Outer mitochondrial membrane (OMM) fusion is catalyzed by the dynamin-like GTPase called mitofusin (MFN). We generated a modified human MFN2 construct with deletions of residues 1–21 and 401–705 (MFN2IM). MFN2IM contains a G domain and a helical domain 1 (HD1). In this study, we address these issues by presenting crystal structures of truncated human MFN2 in different stages of the GTP turnover cycle. These structures explain how MFN2 uses a primate-only single amino acid variance and a tighter G interface, as compared with human MFN1, to allow for enduring GTPase (G) domain association even after GTP hydrolysis, a feature that is unique in the dynamin superfamily and ensures efficient membrane tethering.

To investigate how Thr111 phosphorylation affects the function of MFN2, we solved the crystal structure of a phosphorylation mimic MFN2IM(T111D). According to the structure, the side chain of Asp111 is not fully exposed, and its phosphorylation may require a substantial local conformational rearrangement. Phosphorylated Thr111, as reflected by the Asp111 in the crystal structure, blocks the binding groove for GTP in the P-loop, and the negative charge is also disfavored for the phosphate groups of the nucleotide. Subsequent ITC analysis confirmed that MFN2IM(T111D) has no binding affinity to guanine nucleotides. Therefore, the putative phosphorylation at Thr111 is likely to directly inactivate MFN2 in mediating mitochondrial fusion. Intriguingly, we observed calcium ions (Ca2+) associated with the HD1 of both nucleotide-free wild-type MFN2IM and MFN2IM(T111D), and one of them is involved in intermolecular contact. Addition of Ca2+ did not alter the biochemical features of wild-type MFN2IM or MFN2IM(T111D).

>GPHMGGSAEVNASPLKHFVTAKKKINGIFEQLGAYIQESATFLEDTYRNAELDPVTTEEQVLDVKGYLSKVRGISEVLARRHMKVAFFGRTSNGKSDVINAMLWDKVLPSGIGHTTNCFLRVEGTDGHEAFLLTEGSEEKRSAKTVNQLAHALHQDKQLHAGSLVSVMWPNSKCPLLKDDLVLMDSPGIDVTTELDSWIDKFCLDADVFVLVANSESTLMQTEKHFFHKVSERLSRPNIFILNNRWDASASEPEYMEEVRRQHMERCTSFLVDELGVVDRSQAGDRIFFVSAKEVLNARIQKAQGMPEGGGALAEGFQVRMFEFQNFERRFEECISQSAVKTKFEQHTVRAKQIAEAVRLIMDSLHMAAREQQVYCEEMREERQDRTRENLEQEIAAMNKKIEVLDSLQSKAKLLRNKAGWLDSELNMFTHQYLQPSR[2x]Here, we use human ASNS, a Class II glutamine-dependent amidotransferase that mediates asparagine biosynthesis, as a model system to evaluate whether EM-derived maps can provide insights into conformational changes that might mediate function in multi-site enzymes. As in all other glutamine-dependent enzymes, catalytic turnover requires that ammonia must move through an intramolecular tunnel connecting the active sites. Human ASNS is also of considerable biomedical interest, having been linked to metastatic progression in breast cancer, sarcoma cell proliferation, and decreased effectiveness of clinical treatments for acute lymphoblastic leukemia. Moreover, ASNS variants are strongly correlated with impaired neural development in children, pointing to the importance of gaining an in-depth understanding of how single residue changes might affect activity by altering the conformational preferences and dynamics of the enzyme.

Single-particle images of unmodified, recombinant human ASNS (apo-ASNS) were collected and processed using cryoSPARC62. Data processing (see "Methods") eventually gave rise to a map with 3.5 Å overall resolution. First, two monomers of unmodified human ASNS in the native state form a head-to-head dimer as a result of intermolecular interactions involving residues 31–34 in the adjacent N-terminal domains. The antiparallel orientation of these two peptide segments places the side chains of Arg-32 and Glu-34 in monomer A so that they can form salt bridges with Glu-34 and Arg-32 in monomer B, respectively. Moreover, Phe-31 and Phe-33 in both monomers form a hydrophobic cluster on the other face of the dimerization motif that likely contributes to the stability of the dimer interface in water. Second, the EM and X-ray structures of human ASNS both lack density for residues in two loop segments (residues 201-220 and residues 465-475) and the C-terminal tail (residues 539-560 and 536-560 in the EM and X-ray structures, respectively). As observed for the X-ray structure of DON-modified human ASNS, the intramolecular tunnel in the EM structure adopts a discontinuous, form through which ammonia cannot diffuse. In our overall EM model, Arg-142 adopts a conformation in which the side chain blocks ammonia access to the tunnel, which we therefore designated as closed. In the fifth PC (component 4), the side chain adopts a third conformation, designated as partially open. Closer examination of these structures showed that the carboxylate side chain of Asp-405 formed a salt bridge with Arg-142 when the latter adopted the closed conformation. Based on these findings, we hypothesized that Arg-142 might function as a gate to the ammonia tunnel thereby regulating ammonia translocation between the glutaminase and synthetase active sites.

>[2x]CGIWALFGSDDCLSVQCLSAMKIAHRGPDAFRFENVNGYTNCCFGFHRLAVVDPLFGMQPIRVKKYPYLWLCYNGEIYNHKKMQQHFEFEYQTKVDGEIILHLYDKGGIEQTICMLDGVFAFVLLDTANKKVFLGRDTYGVRPLFKAMTEDGFLAVCSEAKGLVTLKHSATPFLKVEPFLPGHYEVLDLKPNGKVASVEMVKYHHCRDVPLHALYDNVEKLFPGFEIETVKNNLRILFNNAVKKRLMTDRRIGCLLSGGLDSSLVAATLLKQLKEAQVQYPLQTFAIGMEDSPDLLAARKVADHIGSEHYEVLFNSEEGIQALDEVIFSLETYDITTVRASVGMYLISKYIRKNTDSVVIFSGEGSDELTQGYIYFHKAPSPEKAEEESERLLRELYLFDVLRADRTTAAHGLELRVPFLDHRFSSYYLSLPPEMRIPKNGIEKHLLRETFEDSNLIPKEILWRPKEAFSDGITSVKNSWFKILQEYVEHQVDDAMMANAAQKFPFNTPKTKEGYYYRQVFERHYPGRADWLSHYWMPKWINATDPSARTLTHYKSAVKA>[6x]LPSGSDPAFSQPKSVLDAGLTCQGASPSSVSKPILLVPGTGTTGPQSFDSNWIPLSTQLGYTPCWISPPPFMLNDTQVNTEYMVNAITAL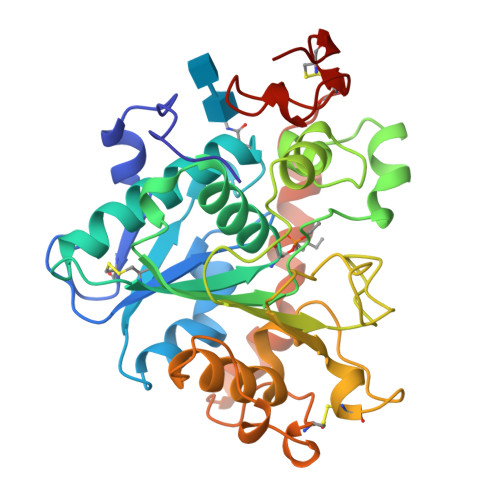YAGSGNNKLPVLTWSQGGLVAQWGLTFFPSIRSKVDRLMAFAPDYKGTVLAGPLDALAVSAPSVWQQTTGSALTTALRNAGGLTQIVPTTNLYSATDEIVQPQVSNSPLDSSYLFNGKNVQAQAVCGPLFVIDHAGSLTSQFSYVVGRSALRSTTGQARSADYGITDCNPLPANDLTPEQKVAAAALLAPAAAAIVAGPKQNCEPDLMPYARPFAVGKRTCSGIVTP> MNKVWDRIVGSDSADAQSVLKERCSSPKDVTDLLHVIQNWTSEIHNNGEETRCWKCVPMLAGYVKDWGQLEFLCRRILLRSSIQEIRPLLLVTMKSLMSNHSDNTEQKCGNILQQLLIEAEEDSGNVSLRLLVDAMSLVFPICLGVCRDMFLSTDFQDILTRNLNSSADDEHLVNGALRLLAVSCIDEAVRRFIAEHYLKTLQQSFKVEKYKVLTALVLIKIWSFTKIEKETLNSCINLFIDSLSNGENIEINTEALAYLTLKPSVRVLLRGNGDVCLKIIELIKSQDTTPTDLYGLLIILANVSEHPSQNEDTVDKLKASLKTNQEKNDEPTLENVKDIEEFNRDYIIDLDLIGSLKSIKLSTSSYNQAIRIIYNVTRDKTQISECVKQGAGLMLLVFLAQKRNLSKDEWYLLSIRALSKTLIYVNPETAFSKYS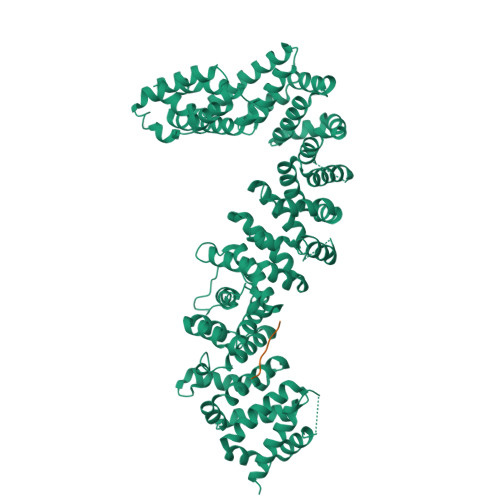PLSAAPFLFENLPLPNDNALSELQFTQLDTYEALLALTNLATINQGVDLGKIILSNAQYWDSIENLLLDSSVRIQRSTLELISNLMSNPMAISAKFFCFENPKSAQNFEILVKLLELHDIQSQRAVAAIFANIASTVPFICKELSEKRNLIETAIRVFKTQNTDTDLRIRLLVLLSSIFNANAHAVACVKNDEEFVKELQKYRNTPSQKDPLTPELSKEILSLINLEHHHHHH;> KFIVSHY>MADKELKFLVVDDFSTMRRIVRNLLKELGFNNVEEAEDGVDALNKLQAGGYGFVISDWNMPNMDGLELLKTIRADGAMSALPVLMVTTEAKKENIIAAAQAGASGYVVKPFTAATLEEKLNK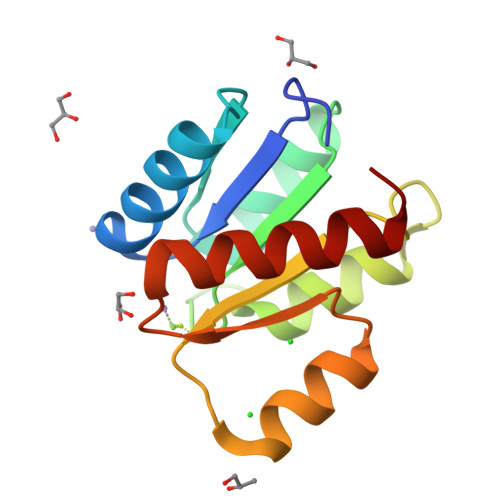IFEKLGM[2x]>HHHHHHMSMKSQFERAKIEYGQWGIDVEEALERLKQVPISIHCAQGDDVGGFELSKGELSGGIDVTGDYPGKATTPEELRMDLEKALSLIPGKHRVNLHAIYAETDGKVVERDQLEPRHFEKWVRWAKRHGLGLDFNPTLFSHEKAKDGLTLAHPDQAIRQFWIDHCIASRKIGEYFGKELETPCLTNIWIPDGYKDTPSDRLTPRKRLKESLDQIFAAEINEAYNLDAVESKLFGIGSESYVVGSHEF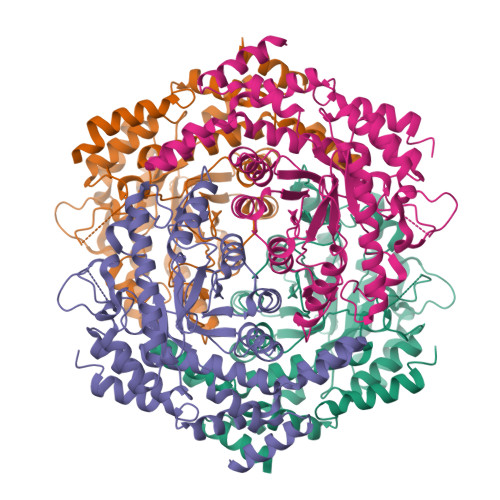YLSYALKNDKLCLLDTGHYHPTETVSNKISAMLLFHDKLALHVSRPVRWDSDHVVTFDDELREIALEIVRNDALDRVLIGLDFFDASINRIAAWTIGTRNVIKALLFAMLIPHKQLKEWQETGDYTRRLAVLEEFKTYPLGAIWNEYCERMNVPIKEEWLKEIAIYEKEVLLQRH[4x]>MNMKTIEDVFIHLLSDTYSAEKQLTRALAK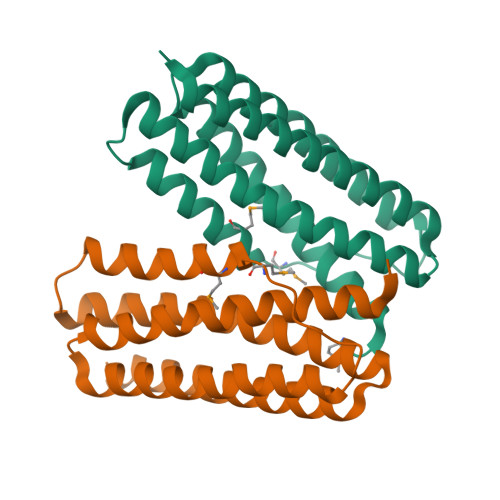LARATSNEKLSQAFHAHLEETHGQIERIDQVVESESNLKIKRMKCVAMEGLIEEANEVIESTEKNEVRDAALIAAAQKVEHYEIASYGTLATLAEQLGYRKAAKLLKETLEEEKATDIKLTDLAINNVNKKAENKA[2x]> MGAAYHFMGKAIPPHQLAIGTLGLLGLLVVPNPFKSAKPKTVDIKTDNKDEEKFIENYLKKHSE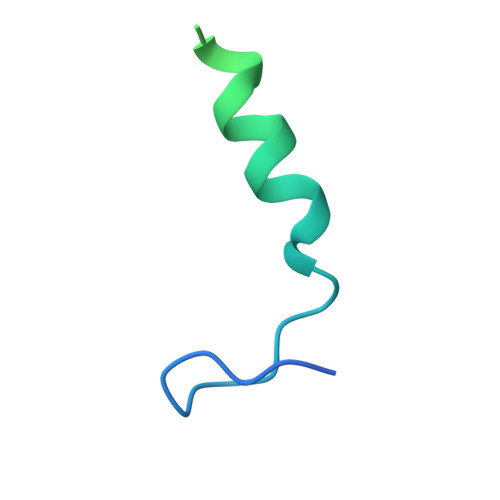KQDA>METSENKSEIKILSLNGGGVRGLFTITLLAELESIIEKREKCENVKIGDYFDLITGTSIGGILALGLASGKSARELKEAFEINATKIFPLKRFKNKQWWNLLRRSIYESEPLYDAVKSMIGETIKFEDLNRRVMITSVNLSTGKPKFFKTPHNPMFTMDREIRLIDAAMATSAAPTYFKPHYIEKLENYFADGGLVANN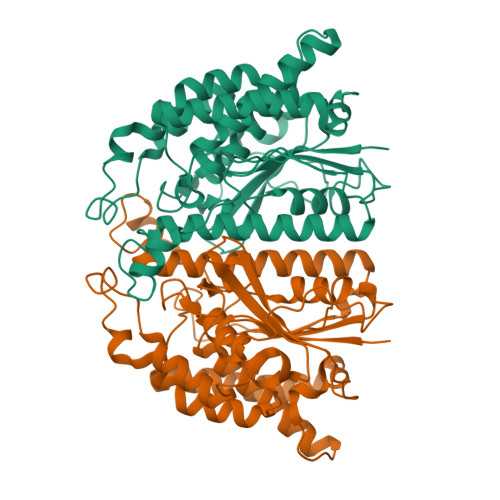PSYIGIREVLIDMKNDFPDAKPENIKVLNIGTLSEDYCISPETLSKNSGKGYLSLWNMGERIVLSTMTANQHLQRFMLLREFEALKIEKNYVEIDETIPNEAAAEITLDNASEGCLKALRGSGKKLAAERYTKNEELRNFFLKKAEPFVPYIESSEVTAHHHHHH[2x]>MATANGAVENGQPDRKPPALPRPIRNLEVKFTKIFINNEWHESKSGKKFATCNPSTREQICEVEEGDKPDVDKAVEAAQVAFQRGSPWRRLDALSRGRLLHQLADLVERDRATLAALETMDTGKPFLHAFFIDLEGCIRTLRYFAG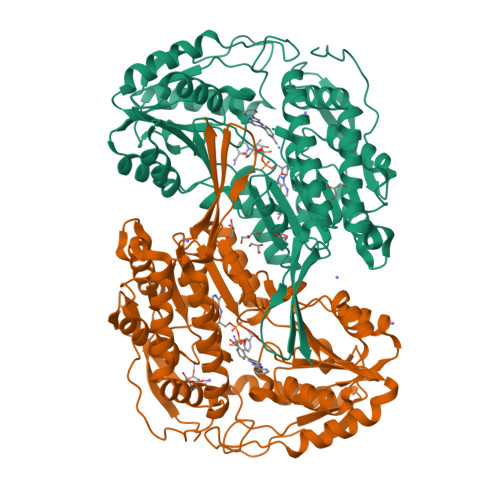WADKIQGKTIPTDDNVVCFTRHEPIGVCGAITPWNFPLLMLVWKLAPALCCGNTMVLKPAEQTPLTALYLGSLIKEAGFPPGVVNIVPGFGPTVGAAISSHPQINKIAFTGSTEVGKLVKEAASRSNLKRVTLELGGKNPCIVCADADLDLAVECAHQGVFFNQGQCCTAASRVFVEEQVYSEFVRRSVEYAKKRPVGDPFDVKTEQGPQIDQKQFDKILELIESGKKEGAKLECGGSAMEDKGLFIKPTVFSEVTDNMRIAKEEIFGPVQPILKFKSIEEVIKRANSTDYGLTAAVFTKNLDKALKLASALESGTVWINCYNALYAQAPFGGFKMSGNGRELGEYALAEYTEVKTVTIKLGDKNP[2x]>[2x]MSSWDVSMSNHAGLVFNPIRTVSDNAKPSPSPKPIIKLSVGDPTLDKNLLTSAAQIKKLKEAIDSQECNGYFPTVGSPEAREAVATWWRNSFVHKEELKSTIVKDNVVLCSGGSHGILMAITAICDAGDYALVPQPGFP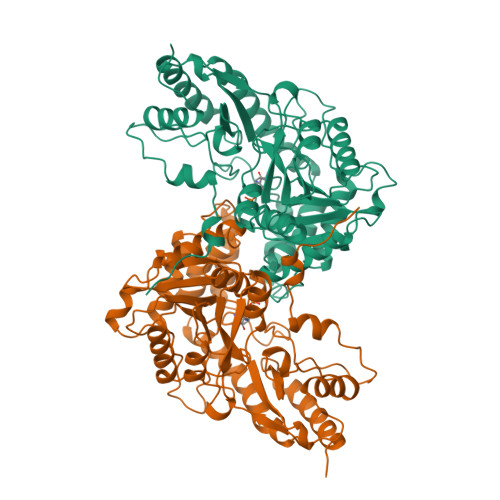HYETVCKAYGIGMHFYNCRPENDWEADLDEIRRLKDDKTKLLIVTNPSNPCGSNFSRKHVEDIVRLAEELRLPLFSDEIYAGMVFKGKDPNATFTSVADFETTVPRVILGGTAKNLVVPGWRLGWLLYVDPHGNGPSFLEGLKRVGMLVCGPCTVVQAALGEALLNTPQEHLDQIVAKIEESAMYLYNHIGECIGLAPTMPRGAMYLMSRIDLEKYRDIKTDVEFFEKLLEEENVQVLPGTIFHAPGFTRLTTTRPVEVYREAVERIKAFCQRHAAV>ARKFYVDQDECIACESCVEIAPGAFAMDPE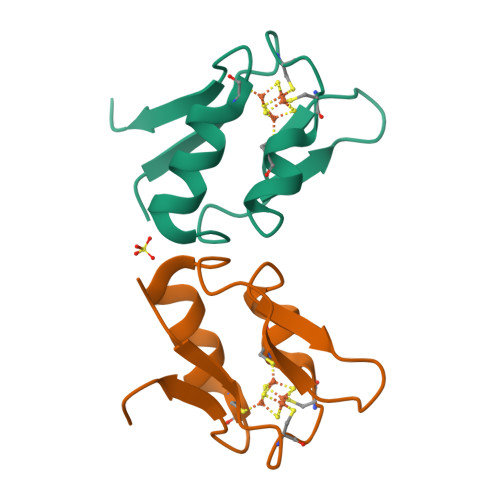IEKAYVKDVEGASQEEVEEAMDTCPVQCIHWEDE[2x]>[2x]AILTGVPYYILPSTSRAGFSPDNLRKNTSQPSCP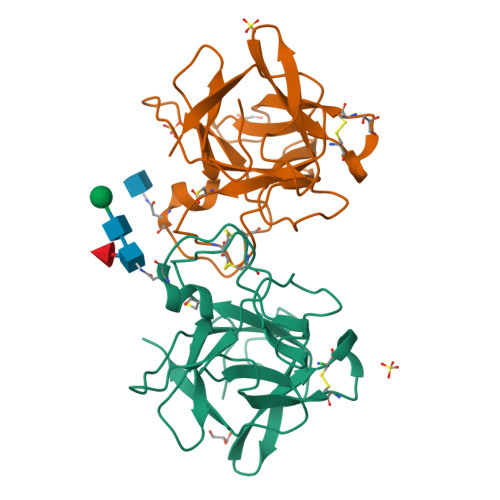LDLITQLRFPPRIGVPVIFTPQNSSLKVVPLSHNLNIHTCSDLWFCPESKIWTVKSSSIHRGLVVTTGGTFRSLGSWFRIERHGDSYKLVHCPRGSTPCRDVGIETVGGGGRRYLAPRDRPLAVRFTRASG> MNKVNVPNFKLNNGDEIPALGYGTWLGVSEKSSGADQPAEEFGFDFDGTDIPKLLDALSYA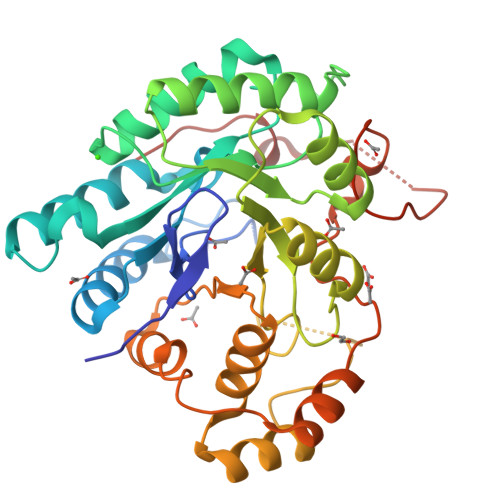IDIGYRHIDTAHFYRVEPEIGQVVQEKINEGVVRREDLFITTKVWQHYHRAADVEVSLRASLHRLGLDHVNLVLMHWPMSISQEGVDEKIDYLETWRGFEEVLKKGLTKAIGVSNFNIEQMKRLLTNCNVPPAVNQIEVNLNLSQADLVDYCQANEVVVVAYSPFGTMVPSRATLNSPEPKLDNPAMLAIGRKYGKTVTQVNLGYLYQRGIVSIPKTVTKSRVLENASIFDFQLDDEDVATLAQFDNGFRTVRPLFWQPYENYPFDVVPGQKHVDIPIAMRKWKNGANGDID>GSHMQCNVPLGMESGRIANEQISASSTYSDGRWTPQQSRLHGDDNGWTPNLDSNKEYLQVDLRFLTMLTAIATQGAISRETQNGYYVKSYKLEVSTNGEDWMVYRHGKNHKVFQANNDATEVVLNKLHAPLLTRFVRIRPQTWHSGIALRLELFGCRVTDAPCSNMLGMLSGLIADSQISAS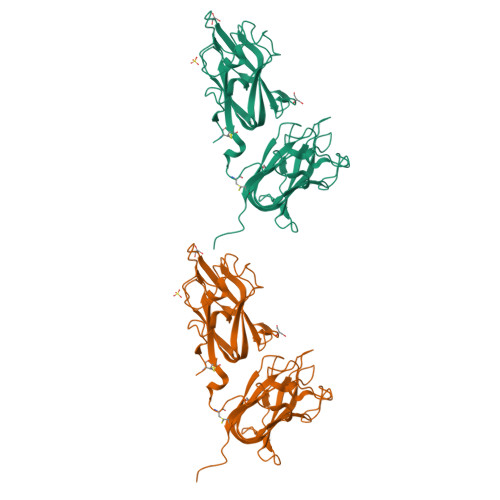STQEYLWSPSAARLVSSRSGWFPRIPQAQPGEEWLQVDLGTPKTVKGVIIQGARGGDSITAVEARAFVRKFKVSYSLNGKDWEYIQDPRTQQPKLFEGNMHYDTPDIRRFDPIPAQYVRVYPERWSPAGIGMRLEVLGCDWTSIIRR[2x]>ARPKLYVMDNGRMRMDKNWMIAMHNPATIHNPNAQTEFVEFPIYTVLIDHPEGKILFDTSCNPNSMGPQGRWAESTQQMFPWTATEECYLHNRLEQLKVRPEDIRYVVASHLHLNHAGCLEMFTNATIIVHEDEFNGALQCYARNQKEGAYIWADIDAWIKNNLQWRTVKRHEDNILLAEGVKVLNFGSGHAWGMLGLHVELPETGGIILASDAIYTAESYGPPIKPPGIIYDSLGYMNTVERIRRIAQETKSQVWFGHDAEQFKKFRKSTEGYYE[3x]

MLLs degrade N-acyl-L-homoserine lactones (AHLs), molecules that are used in a microbial communication system called quorum sensing (QS) to coordinate a variety of behaviors, including virulence and biofilm formation. We provide the structural and biochemical analysis of the lactonase GcL (WP_017434252.1), isolated from the thermophilic bacteria Parageobacillus caldoxylosilyticus. GcL is a thermostable, highly proficient lactonase with broad substrate specificity (kcat/KM values range between 104 to 106 M–1 s–1) for substrates such as N-butyryl (C4) L-homoserine lactone (HSL) and N-decanoyl (C10)-HSL. The binuclear center, common to all MLLs, is coordinated by five histidine residues and two aspartic acid residues.

Asp122 is also conserved and is involved in coordinating the metal cation. To investigate the importance of these residues, we therefore substituted Tyr223 with phenylalanine and Asp122 with asparagine in GcL, eliminating their role in acid catalysis, and kinetically characterized the resulting GcL variants. The alterations in GcL activity may still suggest that this residue is important, but the interpretation of this effect is complicated by the clear role of this residue in metal coordination. This could be seen through crystallization, where multiple conformations were captured: one where both metals are present at high occupancy, exhibiting an active site configuration very similar to that of the wild-type enzyme; and a second form where the active site shows no bound β-metal (or bound with very low occupancy). In the case of the Asp122Asn variant, the Asp mechanism is no longer accessible due to the mutation of Asp122, leaving only the terminal hydroxide or concerted mechanisms as potential options. Curiously, in this variant, the activation free energy for the terminal hydroxide mechanism increases substantially, leaving the concerted mechanism as the only energetically plausible pathway with calculated activation free energies within 3 kcal mol–1 of the experimental data. Visual examination of our EVB trajectories indicates that during our simulations, the substituted N122 side chain interacts with and stabilizes the terminal hydroxide ion at the Michaelis complex, contributing to higher calculated activation free energies through reactant state stabilization.> MLGEDEGNTVLEKGNNPSVKQGEVGAVFIVPKILIREHERVILKQILQILDQDELVQPPLDKFPYKKLELPKYIDELKTRDATNTSYKMIQLDAYGEKKVGSNGELFGGRHYLFNTFTFTAHMGVLLVLLQDVIKVLYQSNATHDEDEFIVQHDQILVMETSEEQTKFLAKNGVIPEESKGSFKYITARSAFVEFGASVIAGGQRIVDDYWESLAKKQNLSSHQRVFKLSTNLISKISLLRPSFQNNRISNANEISANTNNTCTISTSKFESQYPIVTEQPSAEIREAYIENFAKGEHISAIVPGQSISGTLELSAQFRVPRYHSKNSFQQALQMKAMDIPIGRHEELLAQYESQAPDGSASISLPNHIPSVNPSNKPIKRMLSSILDINVSSSKNKKSEENEMIKPM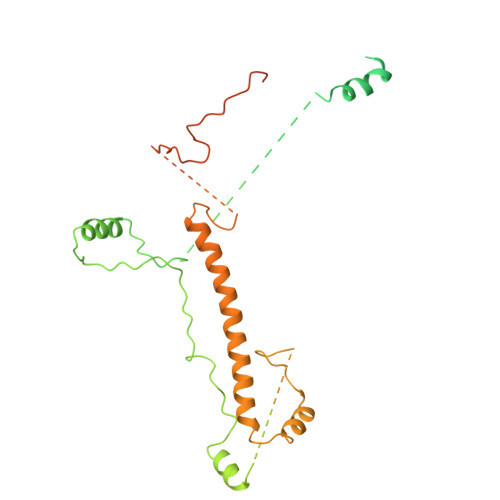NKGQHKNNTSLNINGWKFESLPLKSAENSGKQQYYRGLPLYEKNTLLERLKQLTPNEIKELEHLHDAVFVNTGLQNVRKVRTKKWKKYWQYKAGIPIGLKRSQLDEFKNKYLKDVLAQTSVTTNFNEITNTDETITTKRVPNPNFLGNCNIKDFKPPYIYSHVNKVPQNVAGDKTAVKLDTEVKNTNANPVVATDPVAAKPDNLANFSNEVAMNNGGSGGHHHHHH> YPPSMDWRKKGNFVSPVKNQGSCGSCWTFSTTGALESAV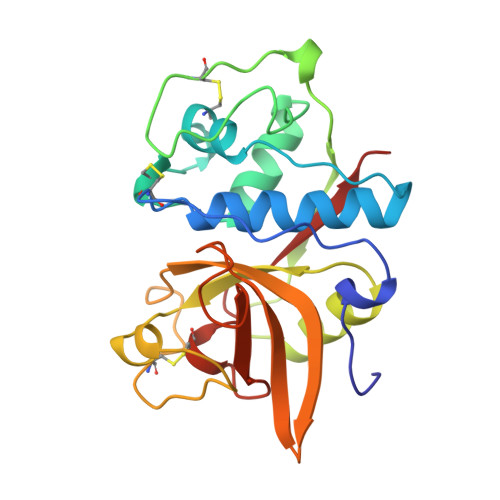AIATGKMLSLAEQQLVDCAQNFNNHGCQGGLPSQAFEYIRYNKGIMGEDTYPYKGQDDHCKFQPDKAIAFVKDVANITMNDEEAMVEAVALYNPVSFAFEVTNDFLMYRKGIYSSTSCHKTPDKVNHAVLAVGYGEENGIPYWIVKNSWGPQWGMNGYFLIERGKNMCGLAACASYPIPLV>MQAEILLTLKLQQKLFADPRRISLLKHIALSGSISQGAKDAGISYKSAWDAINEMNQLSEHILVERATGGKGGGGAVLTRYGQRLIQLYDLL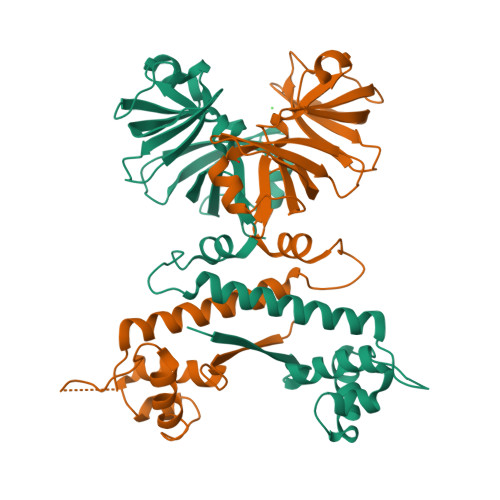AQIQQKAFDVLSDDDALPLNSLLAAISRFSLQTSARNQWFGTITARDHDDVQQHVDVLLADGKTRLKVAITAQSGARLGLDEGKEVLILLKAPWVGITQDEAVAQNADNQLPGIISHIERGAEQCEVLMALPDGQTLCATVPVNEATSLQQGQNVTAYFNADSVIIATLC[4x]> MAHHHHHHMPERMISSSSRSSMSSSTSSEEPLVIDEDFINQVEKHYRKSLKNIPFQYIVGVDVGATNTRIAIQFIINEDQDDEVFMTKFPCNTSTHLANYLAAYGKAMVKAVGKGSAAGSIALAGPVTGDKVRITNYKEHDQEFFYSQLPDTLFPASKNTFLNDLEASCYGIINVGTNNRLHEFFCPIDALNNYATSQTVRLSDTSEYAVLAMGTGLGTGLIVGSAGGKFNVIPLEAGHVHIATPGVNSEHFK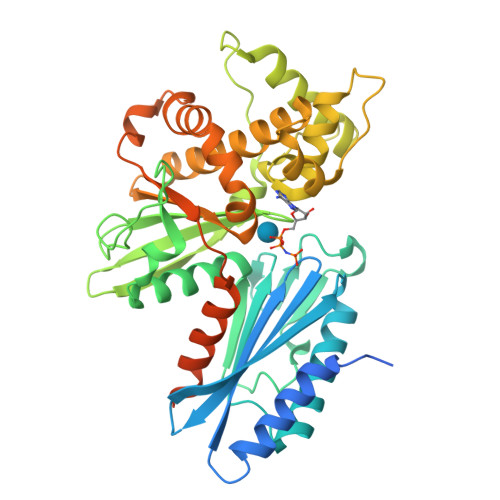EERERIEFLSQKIYGGAYPIEYEDICSGRGLEFCYEFEIRNDPNAVRKTASQIAESYSTDTYARQAMITHYRYLMKAAQNIAVLIPTCRGVFFAGDNQVFNEDFFKEHLSILQKELFQTHQKKHWLTDLKPYRQMKEYNFNVKGCLQKARELAQLGSTTMVDEKPKAGLKDVLSVAIPTAFFSVLSFFTAKNLYEK> NECVSKGFGCLPQSDCPQEARLSYGGCSTVCCDLSKLTGCKGKGGECNPLDRQCKELQAESASCGKGQ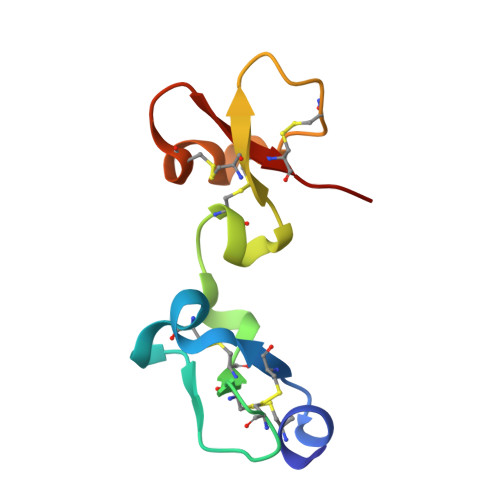KCCVWLH> MDGALINSVLYVSPRNGAHYFVELTEKHLLAFEMLNSMCLLENYDHVLLFLECQFGKSHNLAVIPFDIILVLFTLSTLSEYYKEPILRANDPYNTSRETLSRRALKLLQKYLAILKEFDSEQYNLYDLELLRCQFFLAIDTLTPKKQKWGFDRFRRTKSESGVTYRQNASVDPELDQAKTFKNPYRSYISCLEQRNTILGNRLLNLKLNEPGEFINMILWTLSNSLQESTPLFLSSHEIWMPLLEILIDLFSCRQDYFIQHEVAQNVSKSLFVQRLSESPLAVFFESLNTRNFANRFSEYVFLNCDYKLPSDNYATPVHPVYNGENTIVDTYIPTIKCSPLYKSQKSLALRRKLIGSCFKLLLRVPDGHRLITPRIVADDVIQGISRTLASFNDILQFKKFFMTENLSQESYFIPLLAEGTLSEILKDTQECVVILTLVENLSDGVSFCNEVIGLVKSKCFAFTEQCSQASYEEAVLNIEKCDVCLLVLLRYLLHLIGTEAILDAKEQLEMLHAIEKNDSGRRQWAKALNLG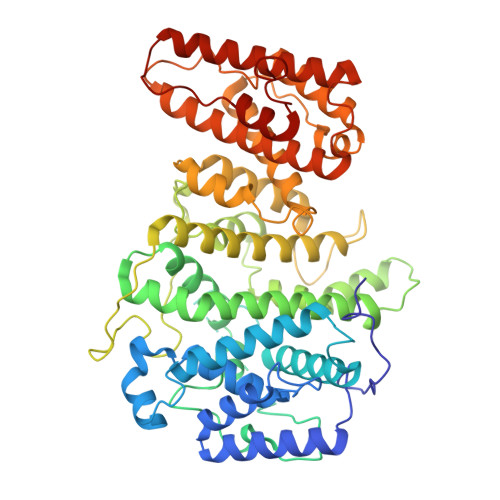NDPPLLYPIVSQMFGVHDKSVIIE> GSHMERPESELIRQSWRVVSRSPLEHGTVLFARL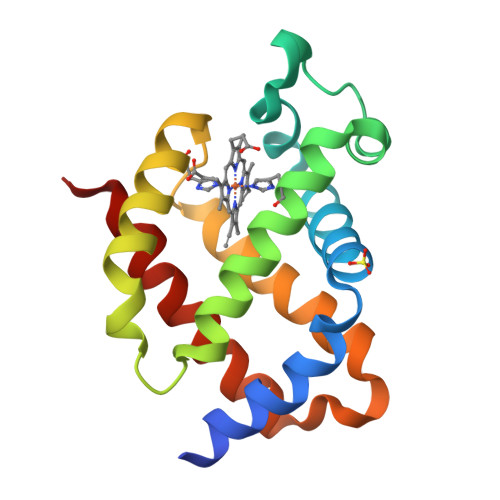FALEPSLLPLFQYNGRQFSSPEDSLSSPEFLDHIRKVMLVIDAAVTNVEDLSSLEEYLTSLGRKHRAVGVRLSSWSTVGESLLYMLEKSLGPDFTPATRTAWSRLYGAVVQAMSRGWDGE> LMYYESLTKQYPVSKTIRNELIPIGKTLDNIRQNNILESDVKRKQNYEHVKGILDEYHKQLINEALDNCTLPSLKIAAEIYLKNQKEVSDREDFNKTQDLLRKEVVEKLKAHENFTKIGKKDILDLLEKLPSISEDDYNALESFRNFYTYFTSYNKVRENLYSDKEKSSTVAYRLINENFPKFLDNVKSYRFVKTAGILADGLGEEEQDSLFIVETFNKTLTQDGIDTYNSQVGKINSSINLYNQKNQKANGFRKIPKMKMLYKQILSDREESFIDEFQSDEVLIDNVESYGSVLIESLKSSKVSAFFDALRESKGKNVYVKNDLAKTAMSNIVFENWRTFDDLLNQEYDLANENKKKDDKYFEKRQKELKKNKSYSLEHLCNLSEDSCNLIENYIHQISDDIENIIINNETFLRIVINEHDRSRKLAKNRKAVKAIKDFLDSIKVLERELKLINSSGQELEKDLIVYSAHEELLVELKQVDSLYNMTRNYLTKKPFSTEKVKLNFNRSTLLNGWDRNKETDNLGVLLLKDGKYYLGIMNTSANKAFVNPPVAKTEKVFKKVDYKLLPVPNQMLPKVFFAKSNIDFYNPSSEIYSNYKKGTHKKGNMFSLEDCHNLIDFFKESISKHEDWSKFGFKFSDTASYNDISEFYREVEKQGYKLTYTDIDETYINDLIERNELYLFQIYNKDFSMYSKGKLNLHTLYFMMLFDQRNIDDVVYKLNGEAEVFYRPASISEDELIIHKAGEEIKNKNPNRARTKETSTFSYDIVKDKRYSKDKFTLHIPITMNFGVDEVKRFNDAVNSAIRIDENVNVIGIDRGERNLLYVVVIDSKGNILEQISLNSIINKEYDIETDYHALLDEREGGRDKARKDWNTVENIRDLKAGYLSQVVNVVAKLVLKYNAIICLEDLNFGFKRGRQKVEKQVYQKFEKMLIDKLNYLVIDKSREQTSPKELGGALNALQLTSKFKSFKELGKQSGVIYYVPAYLTSKIDPTTGFANLFYMKCENVEKSKRFFDGFDFIRFNALENVFEFGFDYRSFTQRACGINSKWTVCTNGERIIKYRNPDKNNMFDEKVVVVTDEMKNLFEQYKIPYEDGRNVKDMIISNEEAEFYRRLYRLLQQTLQMRNSTSDGTRDYIISPVKNKREAYFNSELSDGSVPKDADANGAYNIARKGLWVLEQIRQKSEGEKINLAMTNAEWLEYAQTHLL;> MYYESLTKQYPVSKTIRNELIPIGKTLDNIRQNNILESDVKRKQNYEHVKGILDEYHKQLINEALDNCTLPSLKIAAEIYLKNQKEVSDREDFNKTQDLLRKEVVEKLKAHENFTKIGKKD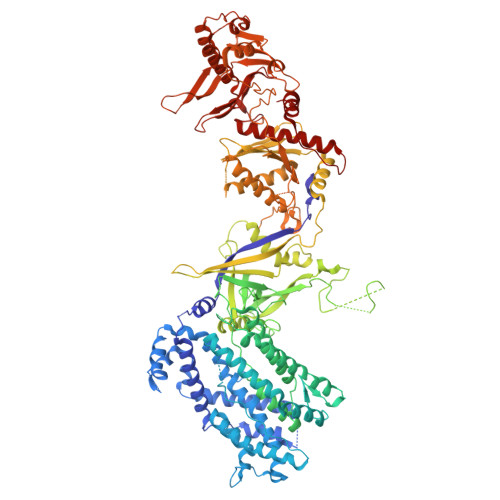ILDLLEKLPSISEDDYNALESFRNFYTYFTSYNKVRENLYSDKEKSSTVAYRLINENFPKFLDNVKSYRFVKTAGILADGLGEEEQDSLFIVETFNKTLTQDGIDTYNSQVGKINSSINLYNQKNQKANGFRKIPKMKMLYKQILSDREESFIDEFQSDEVLIDNVESYGSVLIESLKSSKVSAFFDALRESKGKNVYVKNDLAKTAMSNIVFENWRTFDDLLNQEYDLANENKKKDDKYFEKRQKELKKNKSYSLEHLCNLSEDSCNLIENYIHQISDDIENIIINNETFLRIVINEHDRSRKLAKNRKAVKAIKDFLDSIKVLERELKLINSSGQELEKDLIVYSAHEELLVELKQVDSLYNMTRNYLTKKPFSTEKVKLNFNRSTLLNGWDRNKETDNLGVLLLKDGKYYLGIMNTSANKAFVNPPVAKTEKVFKKVDYKLLPVPNQMLPKVFFAKSNIDFYNPSSEIYSNYKKGTHKKGNMFSLEDCHNLIDFFKESISKHEDWSKFGFKFSDTASYNDISEFYREVEKQGYKLTYTDIDETYINDLIERNELYLFQIYNKDFSMYSKGKLNLHTLYFMMLFDQRNIDDVVYKLNGEAEVFYRPASISEDELIIHKAGEEIKNKNPNRARTKETSTFSYDIVKDKRYSKDKFTLHIPITMNFGVDEVKRFNDAVNSAIRIDENVNVIGIDRGERNLLYVVVIDSKGNILEQISLNSIINKEYDIETDYHALLDEREGGRDKARKDWNTVENIRDLKAGYLSQVVNVVAKLVLKYNAIICLEDLNFGFKRGRQKVEKQVYQKFEKMLIDKLNYLVIDKSREQTSPKELGGALNALQLTSKFKSFKELGKQSGVIYYVPAYLTSKIDPTTGFANLFYMKCENVEKSKRFFDGFDFIRFNALENVFEFGFDYRSFTQRACGINSKWTVCTNGERIIKYRNPDKNNMFDEKVVVVTDEMKNLFEQYKIPYEDGRNVKDMIISNEEAEFYRRLYRLLQQTLQMRNSTSDGTRDYIISPVKNKREAYFNSELSDGSVPKDADANGAYNIARKGLWVLEQIRQKSEGEKINLAMTNAEWLEYAQTHLL> RSSQLPAPQHPKIRLYNAEQVLSWEPVALSNSTRPVVYQVQFKYTDSKWFTADIMSIGVNCTQITATECDFTAASPSAGFPMDFNVTLRLRAELGALHSAWVTMPWFQHYRNVTVGPPENIEVTPGEGSLIIRFSSPFDIADTSTAFFCYYVHYWEKGGIQQVKGPFRSNSISLDNLKPSRVYCLQVQAQLLWNKSNIFRVGHLSNISCYETMADASTELQQTGHHHHHHE

Interferon-γ receptor 2 is a cell-surface receptor that is required for interferon-γ signalling and therefore plays a critical immunoregulatory role in innate and adaptive immunity against viral and also bacterial and protozoal infections. However, to activate this binary complex and activate the JAK/STAT signalization pathway, IFNγ receptor 2 must participate in a ternary complex created by a homodimer of IFNγ, two molecules of receptor 1 and molecule(s) of receptor 2. From its sequence similarity, IFNγ receptor 2 (also known as IFNγ receptor β chain or accessory factor 1, AF-1), has been classified as a member of the class 2 receptor family. It consists of a relatively short 69-amino-acid intracellular domain, a 21-amino-acid transmembrane domain and a 220-amino-acid extracellular domain that is structured into two fibronectin type III domains.

A crystal structure of the extracellular part of human interferon-γ receptor 2 (IFNγR2) was solved by molecular replacement at 1.8 Å resolution. The electron-density map was interpreted for amino-acid residues 28–240, apart from two short loops. The D1 domain is composed of three β-strands stacked on a layer of four β-strands, and the D2 domain is created by four β-strands arranged against four other β-strands; both domains are connected by a short linker (residues 134–143 in IFNγR2) comprising a short helix that is also found in IFNγR1, human tissue factor and other receptors. D1 contains a distinct structural motif of six stacked residues: Lys68, Trp74, Arg114, Trp126, Arg116 and His123. Analysis of the interaction energies in D1 revealed that the motif contributes significantly to the overall stability of the whole domain. A unique feature of IFNγR2 D1 is a short helix (residues 78–85), which is present in no other discussed receptor structure. Our analysis of glycosylation also uncovers the role of the oligosaccharide moieties at Asn110 and Asn137, which sandwich Trp131 and shield its hydrophobic aromatic ring from the solvent. IFNγR2 contains five cysteine residues, and our mass-spectrometric analysis identified disulfide bonds linking Cys86 to Cys94 and Cys209 to Cys234. The fifth IFNγR2 cysteine residue, Cys174, does not form an intramolecular S—S bridge but is bound to a monomeric cysteine.>METFKEYIEKLDKLEFEKMYENDFFLTWEKTRDELEAVFTVADTLRYLRENNISTKIFDSGLGISLFRDNSTRTRFSFASACNLLGLEVQDLDEGKSQISHGETVRETANMISFMADIIGIRDDMYIGKGNAYMHEVSESVQEGYK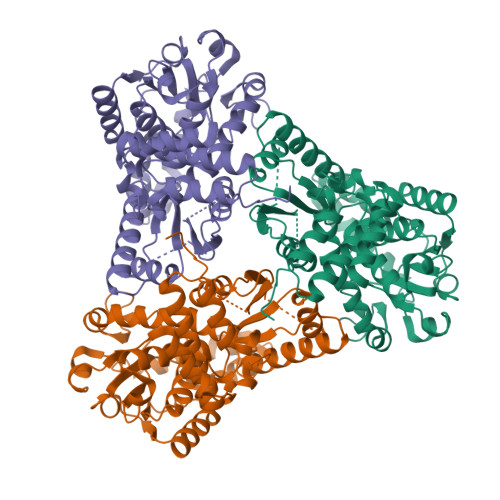DGVLEQRPTLVNLQCDIDHPTQAMADALHLIHEFGGIENLKGKKVAMTWAYSPSYGKPLSVPQGIVGLMTRLGMDVVLAHPEGYEIMPEVEEVAKKNAAEFGGNFTKTNSMAEAFKDADVVYPKSWAPFAAMEKRTELYGNGDQAGIDQLEQELLSQNKKHKDWECTEELMKTTKDGKALYMHCLPADITGVSCEEGEVEASVFDRYRVELYKEASYKPYVIAAMIFLSKVKNPQKTLTDLADKATPREVKDPNSSSVDKLAAALEHHHHHH[2x]>TETTSFLITKFSPDQQNLIFQGDGYTTKEKLTLTKAVKNTVGRALYSSPIHIWDRETGNVANFVTSFTFVINAPNSYNVADGFTFFIAPVDTKPQTGGGYLGVFNSAEYDKTTQTVAVEFDTFYNAAWDPSNRDRHIGIDVNSIKSVNTKSWKLQNGEEANVVIAFNAATNVLTVSLTYPN[2x];>[2x]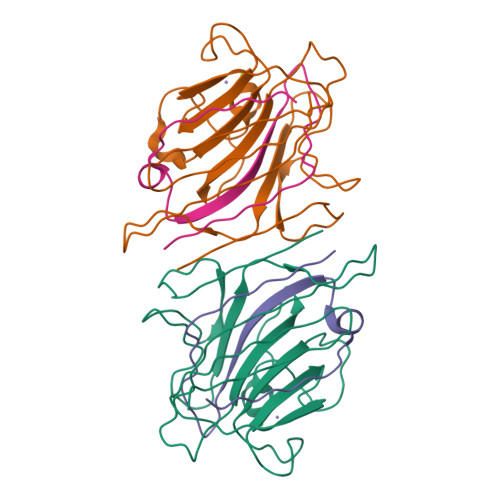VTSYTLSDVVSLKDVVPEWVRIGFSATTGAEYAAHEVLSWSFHSELSGTSSS>MAHHHHHHMKVGILIQARMGSTRLPGKIALPFGDTTILGFMLERLKFSKFQENVVVLTTEENIDDKTEEIAKKNGVSVFRGSANDLIQRYLDAAKTYNIDIIVRLTGDCPLIDSKILDLMVDLFLYNQGRIEFLTNCFQRTFARGMDIEIFTLSLLEKLDSICRLPYEREHIVPYVEENTEKFKFFEYPNERDDSKYRLTIDTIEDYETLKSCISYFLSKEFSYVDLIEVIKKNPSIIQNQTIYHKA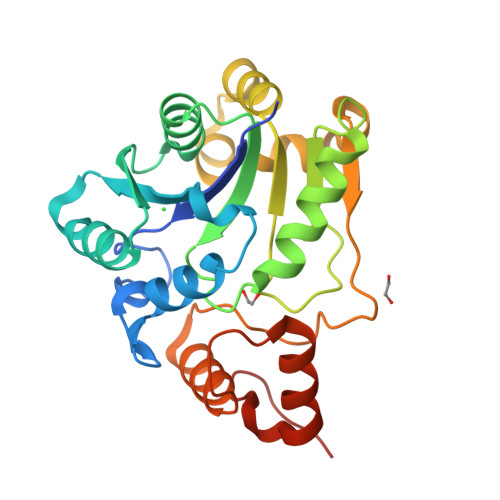YTE[2x]> SPNVEACGYSDRVRQITLGNSTITTQEAANAVVAYGEWPSYLDDKEANPIDAPTEPDVSSNRFYTLDSVQWKSTSRGWWWKLPDALKDMGMF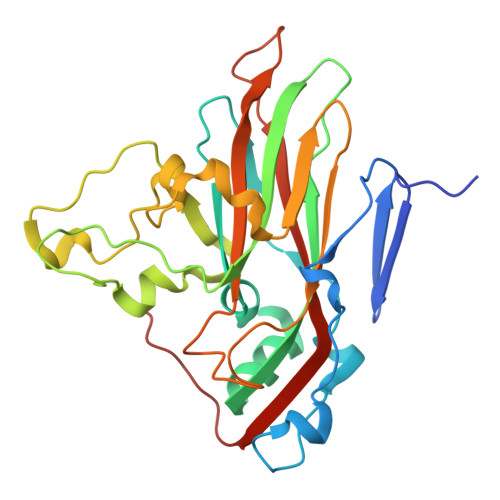GQNMYYHYLGRSGYTVHVQCNASKFHQGALGVFAIPEYVMACNTEAKTSYVSYVNANPGEKGGVFDNAYNPSAEASEGRKFAALDYLLGCGVLAGNAFVYPHQIINLRTNNSATLVLPYVNSLAIDCMAKHNNWGLVILPLCKLDYAPNSSTEIPITVTIAPMFTEFNGLRNITVPATQ>[7x]IDDNDSEKAQKQDIVRVTQTLLDAISCKDFETYTRLCDTSMTCFEPEALGNLIEGIEFHRFYFDGNRKNQVH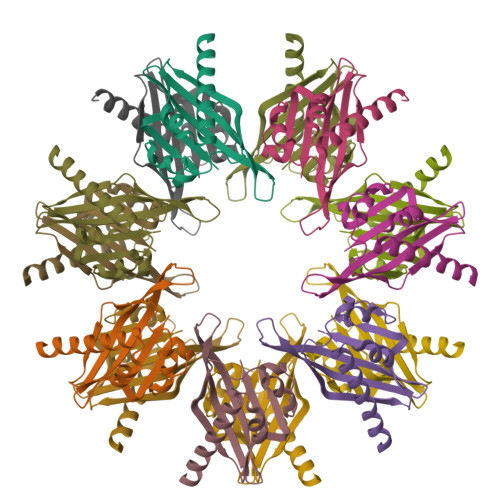TTMLNPNVHIIGEDAACVAYVKLTQFLDRNGEAHTRQSQESRVWSKKQGRWVCVHVHRSTQPSTNTTVSEF> MDAEEKMGVELSSPSAIMEHARRLYMSKDYRSLESLFGRCLKKSYNLDLWMLYIEYVRKVSQKKFKLYEVYEFTLGQFENYWDSYGLYKEYIEEEGKIEDEQTRIEKIRNGYMRALQTPMGSLSELWKDFENFELELNKITGKKIVGDTLPIFQSSFQRYQQIQPLIRGWSVKNAARLIDLEMENGMKLGGRPHESRMHFIHNYILDSFYYAEEVYFFYSEYLIGIGQKEKAKKVVERGIEMSDGMFLSLYYGLVMDEEAVYGDLKRKYSMGEAESAEKVFSKELDLLRINHLNYVLKKRGLELFRKLFIELGNEGVGPHVFIYCAFIEYYATGSRATPYNIFSSGLLKHPDSTLLKEEFFLFLLRIGDEENARALFKRLEKTSRMWDSMIEYEFMVGSMELFRELVDQKMDAIKADAILPPLPPREHNVQMEGILGRYHCFLDSFNFLDLKIRDNSRLLDEFMENLPKISQQNNVLSNLRVEKVISLLKSVQ;> MDAEEKMGVELSSPSAIMEHARRLYMSKDYRSLESLFGRCLWKSYNLDLWMLYIEYVRKVSQKKFKLFEVYEFTLGQFENYWDSYGLFKEYIEELGKIEDEQTRIEKIRNGYMRALQTPMGSLSELWKDFENFELELNKITGKKIVGDTLPLFQSSFQRYQQIQPLIRGWSVKNAARLIDLEMENGMKLGGRPHESRMHFIHNYILDSFFYAEEVYFFYSEYLIGIGQKEKAKKVVERGIEMSDGMFLSLYYGLVMDEEAVYGDLKRKYSMGEAESAEKVFSKELDLLRINHLNYVLKKRGLELFRKLFIELGNEGVGPHVFIYCAFIEYYATGSRATPYNIFSSGLLKHPDSTLLKEEFFLFLLRIGDEENARALFKRLEKTSRMWDSMIEYEFMVGSMELFRELVDQKMDAI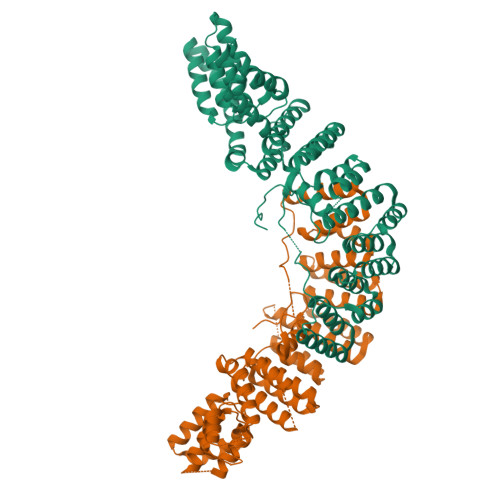KADAILPPLPPREHNVQMEGILGRYHCFLDSFNFLDLKIRDNSRLLDEFMENLPKISQQNNVLSNLRVEKVISLLKSVQ> TAAVALVKANENAAAILNLKNAIQKTNAAVADVVQATQSLGTAVQAVQDHINSVVSPAIT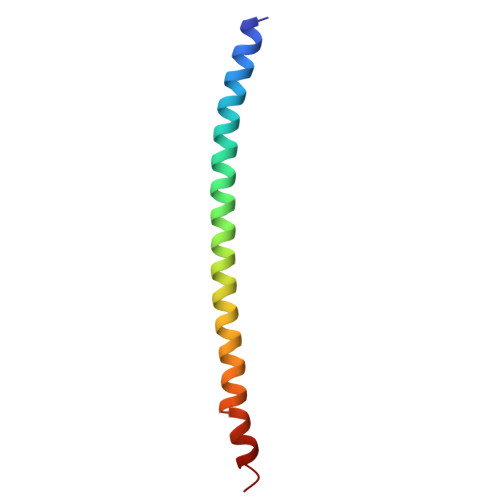AANY> GSSHHHHHHSSGENLYFQHMASWDIFCSVVDNYGDIGVTWRLARQLAAEHGQAVRLWVDEPQAFARICPRADPVAHVQCLDGVEVRAWGRPWAPVAAADVVIEAFACELPEAHRQAMRERKRPSLWLNLEYLSAEEWIGSCHALPSLQACGLSKYFFFPGFREPSGGLLREAGLLERRRRFQASVSAQDEFLASLGVRRKVGERLISLFAYENPALPGWLEQLRDARQPSLLLVPEGRVLADVADWLRVATLAVGDVHVRDALRVQVLPFMA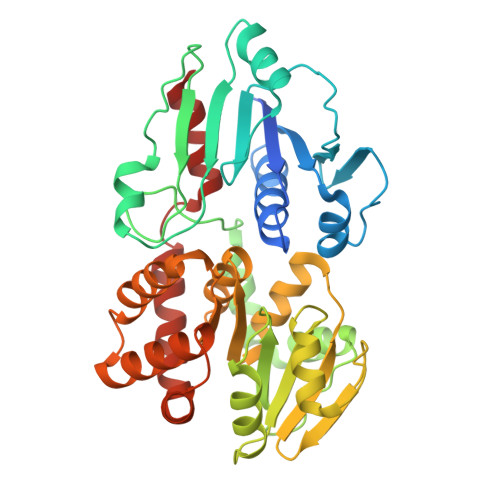QDDYDRLLWCCDLNAVRGEDSFVRAQWAGRPLLWHIYRQEEETHLAKLEAFLELYCAGLPADLAENLRTFWLAWNAGGGLAGAWEGLERQLPEWRREAQRWADEQGMRPDLAARLVQFYADWL(7beta,9beta,13alpha,17beta)-7-{9-[(R)-(4,4,5,5,5-pentafluoropentyl)sulfinyl]nonyl}estra-1(10),2,4-triene-3,17-diol 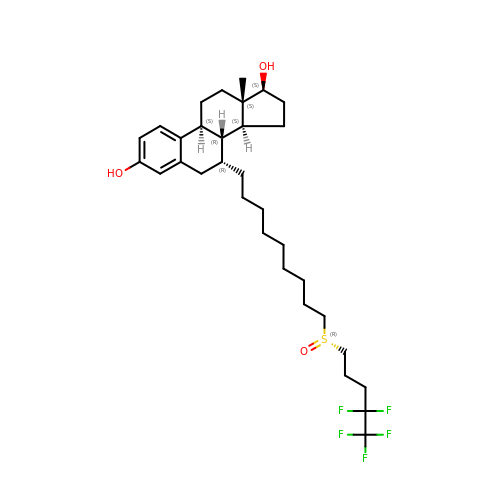| C32 H47 F5 O3 S | VWUXBMIQPBEWFH-CIAKRVSBSA-N>MSLITHFRQAIEETLPWLSSFGADPAGGMTRLLYSPEWLETQQQFKKRMAASGLETRFDEVGNLYGRLNGTEYPQEVVLSGSHIDTVVNGGNLDGQFGALAAWLAIDWLKTQYGAPLRTVEVVAMAEEEGS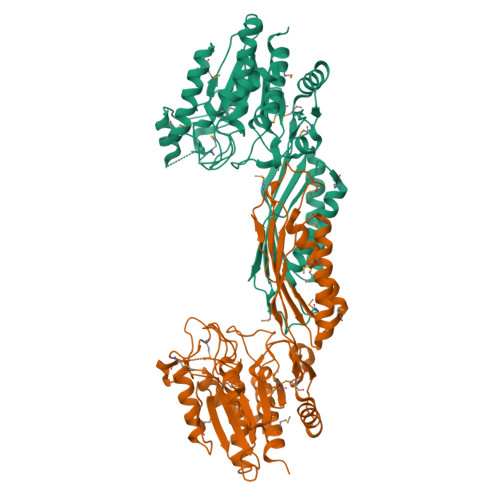RFPYVFWGSKNIFGLANPDDVRNICDAKGNSFVDAMKACGFTLPNAPLTPRQDIKAFVELHIEQGCVLESNGQSIGVVNAIVGQRRYTVTLNGESNHAGTTPMGYRRDTVYAFSRICHQSVEKAKRMGDPLVLTFGKVEPRPNTVNVVPGKTTFTIDCRHTDAAVLRDFTQQLENDMRAICDEMDIGIDIDLWMDEEPVPMNKELVATLTELCEREKLNYRVMHSGAGHDAQIFAPRVPTCMIFIPSINGISHNPAERTNITDLAEGVKTLALMLYQLAWQKEGGSHHHHHH[2x]> KPVPKFRLESLDNPGQFYQADVLTQGKPVLLNVWATWCPTSRAEHQYLNQLSAQGIRVVGMNYKDDRQ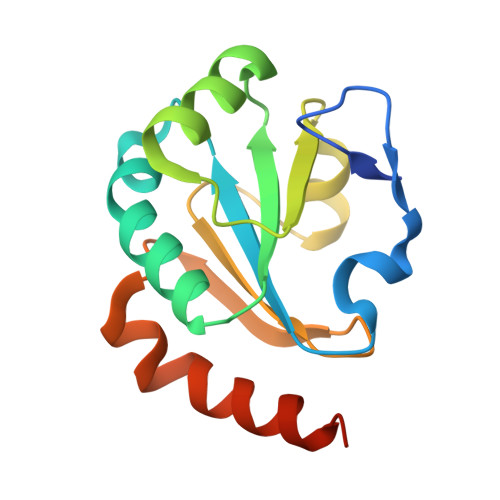KAISWLKELGNPYALSLFDGDGMLGLDLGVYGAPETFLIDGNGIIRYRHAGDLNPRVWEEEIKPLWEKYSKEAAQHHHHHH> MASAVGEKM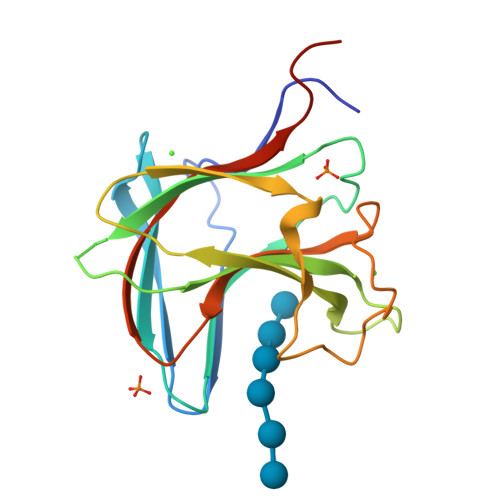LDDFEGVLNWGSYSGEGAKVSTKIVSGKTGNGMEVSYTGTTDGYWGTVYSLPDGDWSKWLKISFDIKSVDGSANEIRFMIAEKSINGVGDGEHWVYSITPDSSWKTIEIPFSSFRRRLDYQPPGQDMSGTLDLDNIDSIHFMYANNKSGKFVVDNIKLIGALEHHHHHH>MAATNMTDNVTLNNDKISGQAWQAMRDIGMSRFELFNGRTQKAEQLAAQAEKLLNDDSTDWNLYVKSDKKAPVEGDHYIRINSSITVAEDYLPAGQKNDAINKANQKMKEGDKKGTIEALKLAGVSVIENQEL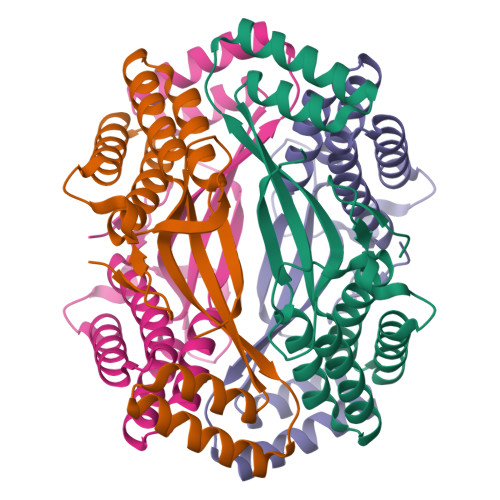IPLQQTRKDVTTALSLMNEGKYYQAGLLLKSAQDGIVVDSQSVQLEHHHHHH[8x]HYDROXY(2-HYDROXYPHENYL)OXOAMMONIUM 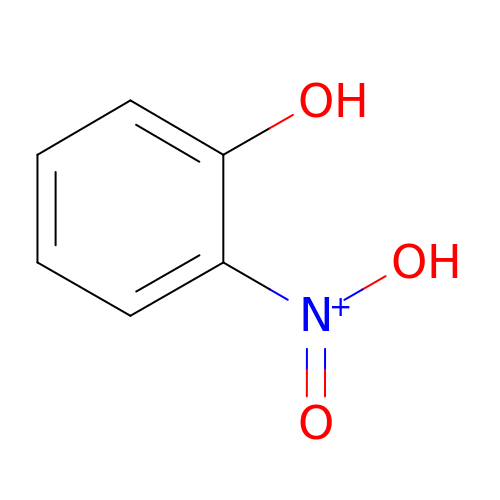| C6 H6 N O3 | CQQWRROYUSGJIU-UHFFFAOYSA-O p-iodo 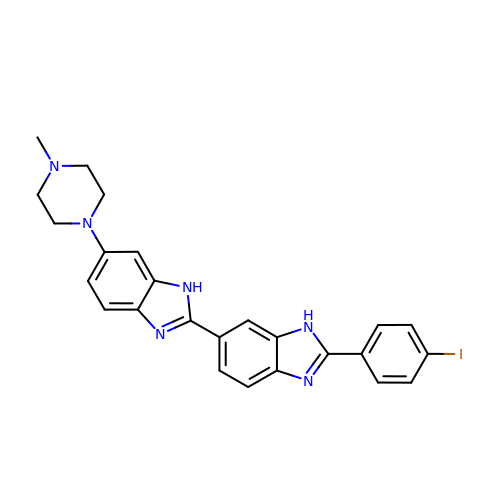Hoechst | C25 H23 I N6 | WSBVZEKIZWIJQO-UHFFFAOYSA-N>[4x]LSSSPSEILQELGKGSTHPQPGVSPPAAPAAPGPKDGPGETDAFGNSEGKELVASGENKIKQGLLPSLEDLLFYTIAEGQEKIPVHKFITALKSTGLRTSDPRLKECMDMLRLTLQTTSDGVMLDKDLF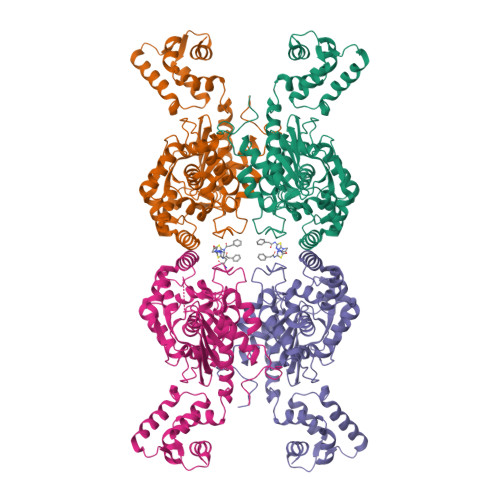KKCVQSNIVLLTQAFRRKFVIPDFMSFTSHIDELYESAKKQSGGKVADYIPQLAKFSPDLWGVSVCTVDGQRHSTGDTKVPFCLQSCVKPLKYAIAVNDLGTEYVHRYVGKEPSGLRFNKLFLNEDDKPHNPMVNAGAIVVTSLIKQGVNNAEKFDYVMQFLNKMAGNEYVGFSNATFQSERESGDRNFAIGYYLKEKKCFPEGTDMVGILDFYFQLCSIEVTCESASVMAATLANGGFCPITGERVLSPEAVRNTLSLMHSCGMYDFSGQFAFHVGLPAKSGVAGGILLVVPNVMGMMCWSPPLDKMGNSVKGIHFCHDLVSLCNFHNYDNLRHFAKKLDPRREGGDQRHSFGPLDYESLQQELALKETVWKKVSPESNEDISTTVVYRMESLGEKS>MDLLTAKTIVLGCSAVGAGLAMIAGLGPGIGEGYAAGKAVESVARQPEARGSIISTMILGQAVAESTGIYSLVIALILLYANPFLSKLG[22x]

In the Fo sector, eight to 15 copies of subunit c are assembled into a closed ring, which rotates around its axis as ions permeate across the enzyme. The c-ring harbors a series of identical ion-binding sites, typically one per c-subunit, which selectively recognize the coupling ion. We describe the structure of a novel type of Na+-binding site in the c-ring of the F1Fo-ATP synthase from F. nucleatum and demonstrate that this enzyme is physiologically coupled to the SMF. The c-ring features two glutamate residues in each of its 11 ion-binding sites, instead of a single carboxylate side-chain as is typical.

We also investigated the influence of the environmental pH on the conformational state of the ion-binding site, by crystallizing the F. nucleatum c11 ring in NaOH-titrated buffer at pH 8.7. The resulting structure, at 2.6 Å resolution, revealed again a locked conformation of the binding site identical to that at pH 5.3, with Na+ and H+ bound concurrently. As we observed in previous structural studies of c-rings, the detergent used in these crystals provides a hydrophobic belt that effectively uncouples the binding sites from the pH or Na+ concentration conditions in the crystallization buffer, in a manner that likely resembles the shielding effect of a lipid membrane. The finding that one Na+ and one H+ can concurrently occupy the binding sites in the F. nucleatum c11 ring raises the possibility that both ions are co-transported across the membrane as the ring rotates. In sum, computations and measurements demonstrate that the protons that occupy the ion-binding sites in the F. nucleatum c-ring, concurrently with Na+, remain bound to the structure throughout the rotation of the ring, and therefore are not co-translocated with Na+ across the membrane.Disulfide-bond-forming protein A (DsbA) catalyzes the formation of the disulfide bonds necessary for the activity and stability of multiple substrate proteins, including many virulence factors. DsbA works in tandem with its membrane-embedded partner protein DsbB, which is required to maintain DsbA in its active, oxidized state. B. pseudomallei is a Gram-negative bacterium that is found predominantly in tropical areas and is the causative agent of the deadly disease melioidosis. Binding was characterized using NMR and X-ray crystallo­graphy. Both 1 and 2 bind to a transient (or ‘cryptic’) pocket on BpsDsbA located adjacent to the redox active site which is not observed in the apo BpsDsbA structure.

Oxidized BpsDsbA was co-crystallized with 1 in 60% Tacsimate (Hampton Research); the resulting crystals diffracted to a resolution of 1.84 Å on beamline MX2 at the Australian Synchrotron and belonged to space group P212121. The interactions between 1 and the protein are mostly hydrophobic, involving the side chains of Tyr110, Trp40, Phe77 and Leu112 from the original copy of the protein and Val12, Ala13 and Lys15 of the next symmetry-related protein molecule in the crystal. Additionally, there are π-stacking interactions between the aromatic rings of the fragment and Tyr110 (4.1 Å, measured from the centroid of each ring). The fragment binds within 10 Å of the redox active-site residue Cys43. During refinement of the structure, the optimal occupancy of fragment 1 was found to be 0.62, suggesting that the observed density reflects a mixture of the apo and fragment-bound forms of the protein in the crystal. The signal was particularly intense for the Br atom, where difference density was visible even above the 20 r.m.s.d. level. Two additional residues, Ala72 and Lys108, showed a CSP of >0.02 p.p.m. for 1.

> SNAAGFAQASPSAPVAGKDFEVMKSPQPVSAPAGKVEVIEFFWYGCPHCYEFEPTIEAWVKKQGDKIAFKRVPVAFRDDFVPHSKLFYALAALGVSEKVTPAVFNAIHKEKNYLLTPQAQADFLATQGVDKKKFLDAYNSFSVQGQVKQSAELLKNYNIDGVPTIVVQGKYKTGPAYTNSLEGTAQVLDFLVKQVQDKKL>QLPTIYAITPTYSRPVQKAELTRLANTFRQVAQLHWILVEDAAARSELVSRFLARAGLPSTHLHVPTPRRYKRPGLPRATEQRNAGLAWLRQRHQH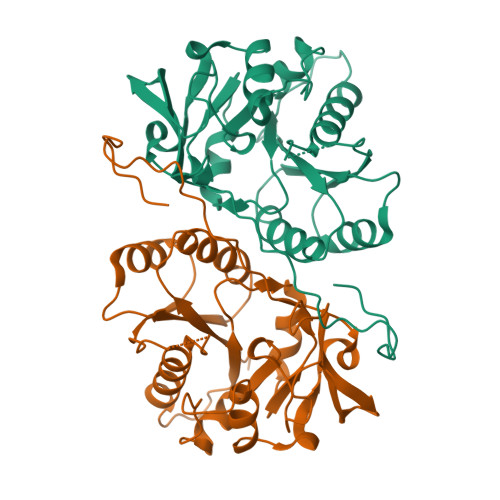QRAQPGVLFFADDDNTYSLELFQEMRTTRKVSVWPVGLVGGRRYERPLVENGKVVGWYTGWRADRPFAIDMAGFAVSLQVILSNPKAVFKRRGSQPGMQESDFLKQITTVEELEPKANNCTKVLVWHTRTEKVNLANEPKYHLDTVKIEV[4x]> AAGAAPVDISTLPRVKVDLVKPPFV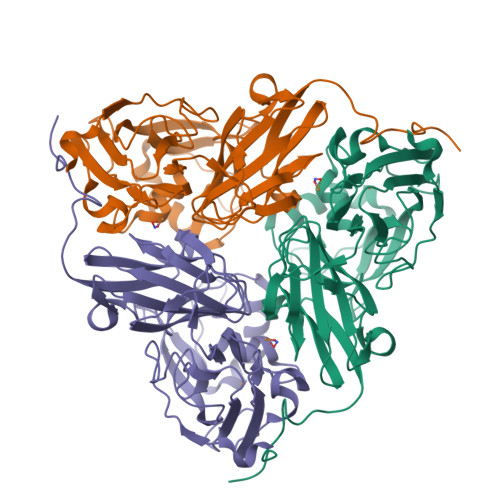HAHDQVAKTGPRVVEFTMTIEEKKLVIDREGTEIHAMTFNGSVPGPLMVVHENDYVELRLINPDTNTLLHNIDFHAATGALGGGALTQVNPGEETTLRFKATKPGVFVYHCAPEGMVPWHVTSGMNGAIMVLPRDGLKDEKGQPLTYDKIYYVGEQDFYVPKDEAGNYKKYETPGEAYEDAVKAMRTLTPTHIVFNGAVGALTGDHALTAAVGERVLVVHSQANRDTRPHLIGGHGDYVWATGKFRNPPDLDQETWLIPGGTAGAAFYTFRQPGVYAYVNHNLIEAFELGAAGHFKVTGEWNDDLMTSVVKPASM> PMVMWKDLLTGSWKGPDVLITA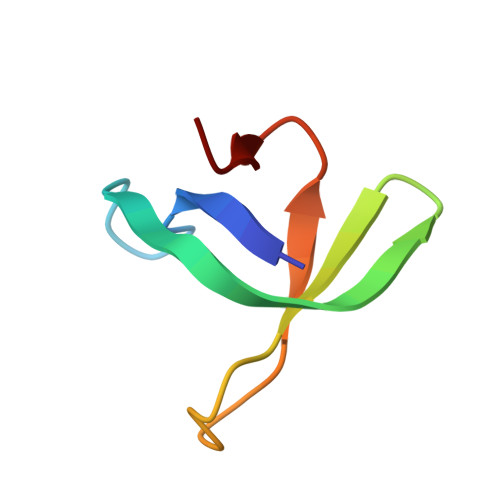GRGYACVFPQDAESPIWVPDRFIRPFT> GSMFGCLVAGRLVQTAAQQVAEDKFVFDLPDYESINHVVVFMLGTIPFPEG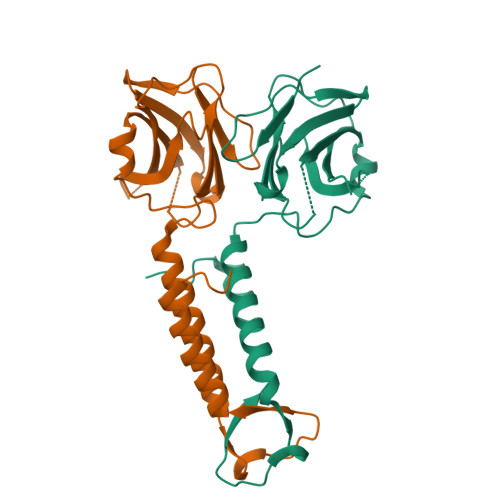MGGSVYFSYPDSNGMPVWQLLGFVTNGKPSAIFKISGLKSGEGSQHPAGAMNIVRTPSVAQIGISVELLDSMAQQTPVGNAAVSSVDSFTQFTQKMLDNFYNFASSFAVSQAQMTPSPSEMFIPANVVLKWYENFQRRLAQNPLFWKT;> SMFGCLVAGRLVQTAAQQVAEDKFVFDLPDYESINHVVVFMLGTIPFPEGMGGSVYFSYPDSNGMPVWQLLGFVTNGKPSAIFKISGLKSGEGSQHPAGAMNIVRTPSVAQIGISVELLDSMAQQTPVGNAAVSSVDSFTQFTQKMLDNFYNFASSFAVSQAQMTPSPSEMFIPANVVLKWYENFQRRLAQNPLFWKT>[2x]MSKKKFVIVSILTILLVQAIYFVEKYHTSEDKSTSNTSSTPPQTTLSTTKVLKIRYPDDGEWPGAPIDKDGDGNPEFYIEINLWNILNATGFAEMTYNLTSGVLHYVQQLDNIVLRDRSNWVHGYPEIFYGNKPWNANYATDGPIPLPSKVSNLTDFYLTISYKLEPKNGLPINFAIESWLTREAWRTTGINSDEQEVMIWIYYDGL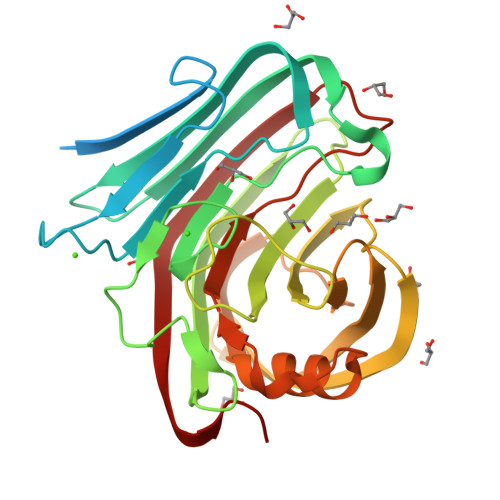QPAGSKVKEIVVPIIVNGTPVNATFEVWKANIGWEYVAFRIKTPIKEGTVTIPYGAFISVAANISSLPNYTELYLEDVEIGTEFGTPSTTSAHLEWWITNITLTPLDRPLIS[3-bromo-5-(pyrrolidin-1-yl)phenyl]borinic acid | C10 H13 B Br N O | 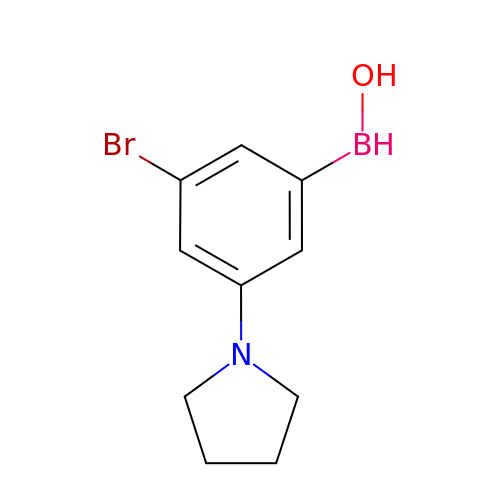NSKSGJKZESIODM-UHFFFAOYSA-N DyPs (dye-decolorizing peroxidases) (EC 1.11.1.19) represent a new family of haem peroxidases widespread in bacteria, archaea, fungi and other micro-organisms. In the present study, we expressed A. auricula-judae DyP in E. coli, solved the crystal structure of the recombinant enzyme and several site-directed variants, and used PELE (Protein Energy Landscape Exploration) to describe the binding of its typical substrate RB19. The DyP structure is formed by two domains, each of them including an antiparallel four-stranded large β-sheet and two or three helices resulting in a ferredoxin-like fold (plus two additional β-strands). In spite of the obvious similarity between the two domains, only the C-terminal domain harbours a haem cofactor.

At the opposite side of the haem, Asp-168 and Arg-332 occupy neighbouring positions, suggesting a contribution to the haem reaction with H2O2. Then, the exposed aromatic residues identified in PELE and QM/MM simulations were substituted to verify their eventual involvement in catalysis (information on the effect of mutating haem pocket residues is provided in the Supplementary Results). Moreover, most of the variants show crystal structures largely superimposable with that of WT DyP, except for the mutated residues. The EPR spectrum of the WT DyP resting state (top) shows a ferric species prevalently in its axial high spin state (g⊥≈ 6 and g∥=2.0). After adding 10 eq. of H2O2, a strong decrease in the ferric signal, and appearance of an intense protein radical signal are evident (bottom) (the electronic absorption spectra of WT DyP, and the EPR and electronic absorption spectra of the D168N and R332L variants are described in the Supplementary Results and Supplementary Figures S4 and S5 respectively).

>[2x]MATSLNTIDIQGDILVGMHKQKQLFYFFAINDPATFKTHLASDIAPVVASVTQLSNVATQPLVALNIAFSNTGLLALGVTDNLGDSLFANGQAKDATSFKESTSSWVPQFAGTGIHGVIILASDTTDLIDQQVASIESTFGSSISKLYSLSASIRPGNEAGHEMFGFLNGIAQPAINGFNTPLPGQNIVDAGVIITGATNDPITRPSWAVGGSFLAFRQLEQLVPEFNKYLLDNAPAGSGSLQARADLLGARMVGRWKSGAPIDLTPTADDPALGADAQRNNNFTYSHAGFDLGSDQSHCPFSAHIRKTRPRADLGGSLTPPNLSAGANSIMRSGIPYGPEVTSAESASNTTTQERGLAFVAYQAQLSQGFHFLQQTWADNANFPPGKTPATVGLDPIIGQNNGQPRVVNGLLPSNSSASLSIPQFVVSHGGEYFFSPPISAIGGRLSA>PKTQRGIYHNLKESEYVASNTDVTFFFSSELYLNKFLDGYQEYRKKFNKKIERVAVTPWNMDMLADIT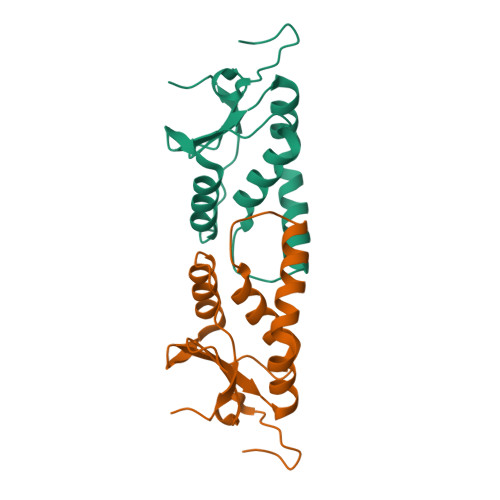FYSEVEKRGFHAWLKGDNATWREVHVYALRIMTKPNTLDWSRIQKPR[6x]> MAKDIEISASESKFILEALRQNYRLDGRSFDQFRDVEITFGKEFGDVSVKMGNTKVHCRISCQIAQPYEDRPFEGLFVISTEISPMAGSQFENGNITGEDEVLCSRIIEKSVRRSGALDVEGLCIVAGSKCWAVRADVHFLDCDGGFIDASCIAVMAGLMHFKKPDITVHGEQIIVHPVNEREPVPLGILHIPICVTFSFFNPQDTEENIKGETNSEISIIDATLKEELLRDGVLTVTLNKNREVVQVSKAGGLPMDALTLMKCCHEAYSIIEKITDQILQLLKEDSEKRNKYAAMLTSENAREI;> GHMSRLEIYSPEGLRLDGRRWNELRRFESSINTHPHAADGSSYMEQGNNKIITLVKGPKEPRLKSQMDTSKALLNVSVNITKFSKFERSKSSHKNERRVLEIQTSLVRMFEKNVMLNIYPRTVIDIEIHVLEQDGGIMGSLINGITLALIDAGISMFDYISGISVGLYDTTPLLDTNSLEENAMSTVTLGVVGKSEKLSLLLVEDKIPLDRLENVLAIGIAGAHRVRDLMDEELRKHAQKRVSNASAR;> MAESTTLETIEIHPITFPPEVLARISPELSLQRHLSLGIRPCLRKYEEFRDVAIENNTLSRYADAGNIDTKNNILGSNVLKSGKTIVITSITGGIIEETSASIKDLDDFGEEELFEVTKEEDIIANYASVYPVVEVERGRVGACTDEEMTISQKLHDSILHSRILPKKALKVKAGVRSANEDGTFSVLYPDELEDDTLNETNLKMKRKWSYVLYAKIVVLSRTGPVFDLCWNSLMYALQSVKLPRAFIDERASDLRMTIRTRGRSATIRETYEIICDQTKSVPLMINAKNIAFASNYGIVELDPECQLQNSDNSEEEEVDIDMDKLNTVLIADLDTEAEETSIHSTISILAAPSGNYKQLTLMGGGAKITPEMIKRSLLLSRVRADDLSTRFNI;> GHGNNKEPNTKNRLDSAEKKKKMSVQAEIGILDHVDGSSEFVSQDTKVICSVTGPIEPKARQELPTQLALEIIVRPAKGVATTREKVLEDKLRAVLTPLITRHCYPRQLCQITCQILESGEDEAEFSLRELSCCINAAFLALVDAGIALNSMCASIPIAIIKDTSDIIVDPTAEQLKISLSVHTLALEFVNGGKVVKNVLLLDSNGDFNEDQLFSLLELGEQKCQELVTNIRRIIQDNISPRLVV;> GHMSLSVAEKSYLYDSLASTPSIRPDGRLPHQFRPIEIFTDFLPSSNGSSRIIASDGSECIVSIKSKVVDHHVENELLQVDVDIAGQRDDALVVETITSLLNKVLKSGSGVDSSKLQLTKKYSFKIFVDVLVISSHSHPISLISFAIYSALNSTYLPKLISAFDDLEVEELPTFHDYDMVKLDINPPLVFILAVVGNNMLLDPAANESEVANNGLIISWSNGKITSPIRSVALNDSNVKSFKPHLLKQGLAMVEKYAPDVVRSLENL;> MNVQDRRRLLGPAAAKPMAFSNTTTHVPEKKSTDLTPKGNESEQELSLHTGFIENCNGSALVEARSLGHQTSLISAVYGPRSIRGSFTSQGTISIQLKNGLLEKYNTNELKEVSSFLMGIFNSVVNLSRYPKSGIDIFVYLTYDKDLTNNPQDDDSQSKMTSSQISSLIPHCITSITLALADAGIELVDMAGAGEANGTVVSFIKNGEEIVGFWKDDGDDEDLLECLDRCKEQYNRYRDLMISCLMNQET;> GPHMSTFIFPGDSFPVDPTTPVKLGPGIYCDPNTQEIRPVNTGVLHVSAKGKSGVQTAYIDYSSKRYIPSVNDFVIGVIIGTFSDSYKVSLQNFSSSVSLSYMAFPNASKKNRPTLQVGDLVYARVCTAEKELEAEIECFDSTTGRDAGFGILEDGMIIDVNLNFARQLLFNNDFPLLKVLAAHTKFEVAIGLNGKIWVKCEELSNTLACYRTIMECCQKNDTAAFKDIAKRQFKEILTVKEE;> RSMSEVITITKRNGAFQNSSNLSYNNTGISDDENDEEDIYMHDVNSASKSESDSQIVTPGELVTDDPIWMRGHGTYFLDNMTYSSVAGTVSRVNRLLSVIPLKGRYAPETGDHVVGRIAEVGNKRWKVDIGGKQHAVLMLGSVNLPGGILRRKSESDELQMRSFLKEGDLLNAEVQSLFQDGSASLHTRSLKYGKLRNGMFCQVPSSLIVRAKNHTHNLPGNITVVLGVNGYIWLRKTSQMDLARDTPSANNSSSIKSTGPTGAVSLNPSITRLEEESSWQIYSDENDPSISNNIRQAICRYANVIKALAFCEIGITQQRIVSAYEASMVYSNVGELIEKNVMESIGSDILTAEKMRGNGN;> GPHMACNFQFPEIAYPGKLICPQYGTENKDGEDIIFNYVPGPGTKLIQYEHNGRTLEAITATLVGTVRCEEEKKTDQEEEREGTDQSTEEEKSVDASPNDVTRRTVKNILVSVLPGTEKGRKTNKYANNDFANNLPKEGDIVLTRVTRLSLQRANVEILAVEDKPSPIDSGIGSNGSGIVAAGGGSGAATFSVSQASSDLGETFRGIIRSQDVRSTDRDRVKVIECFKPGDIVRAQVLSLGDGTNYYLTTARNDLGVVFARAANGAGGLMYATDWQMMTSPVTGATEKRKCAKPF;> GPAMSVPAIAPRRKRLADGLSVTQKVFVRSRNGGATKIVREHYLRSDIPCLSRSCTKCPQIVVPDAQNELPKFILSDSPLELSAPIGKHYVVLDTNVVLQAIDLLENPNCFFDVIVPQIVLDEVRNKSYPVYTRLRTLCRDSDDHKRFIVFHNEFSEHTFVERLPNETINDRNNRAIRKTCQWYSEHLKPYDINVVLVTNDRLNREAATKEVESNIITKSLVQYIELLPNADDIRDSIPQMDSFDKDLERDTFSDFTFPEYYSTARVMGGLKNGVLYQGNIQISEYNFLEGSVSLPRFSKPVLIVGQKNLNRAFNGDQVIVELLPQSEWKAPSSIVLDSEHFDVNDNPDIEAGDDDDNNESSSNTTVISDKQRRLLAKDAMIAQRSKKIQPTAKVVYIQRRSWRQYVGQLAPSSVD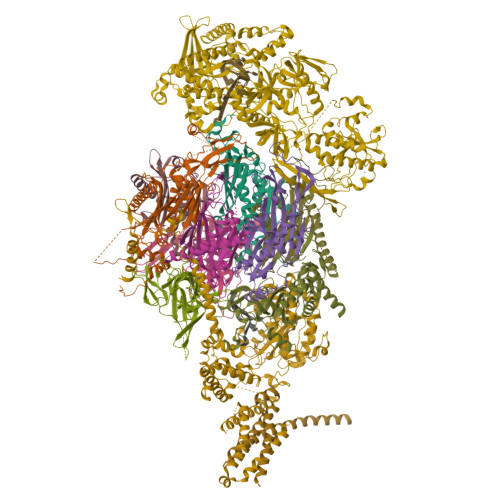PQSSSTQNVFVILMDKCLPKVRIRTRRAAELLDKRIVISIDSWPTTHKYPLGHFVRDLGTIESAQAETEALLLEHDVEYRPFSKKVLECLPAEGHDWKAPTKLDDPEAVSKDPLLTKRKDLRDKLICSIDPPGCVDINDALHAKKLPNGNWEVGVHIADVTHFVKPGTALDAEGAARGTSVYLVDKRIDMLPMLLGTDLCSLKPYVDRFAFSVIWELDDSANIVNVNFMKSVIRSREAFSYEQAQLRIDDKTQNDELTMGMRALLKLSVKLKQKRLEAGALNLASPEVKVHMDSETSDPNEVEIKKLLATNSLVEEFMLLANISVARKIYDAFPQTAMLRRHAAPPSTNFEILNEMLNTRKNMSISLESSKALADSLDRCVDPEDPYFNTLVRIMSTRCMMAAQYFYSGAYSYPDFRHYGLAVDIYTHFTSPIRRYCDVVAHRQLAGAIGYEPLSLTHRDKNKMDMICRNINRKHRNAQFAGRASIEYYVGQVMRNNESTETGYVIKVFNNGIVVLVPKFGVEGLIRLDNLTEDPNSAAFDEVEYKLTFVPTNSDKPRDVYVFDKVEVQVRSVMDPITSKRKAELLLK;> GAMASENPDVLLSRVINVVRAASSLASQDVDFYKNLDRGFSKDLKSKADKLADMANEIILSIDEHHESFELKEEDISDLWNNFGNIMDNLLEMSDHSLDKLNCAINSKSRGSDLQYLGEFSGKNFSPTKRVEKPQLKFKSPIDNSESHPFIPLLKEKPNALKPLSESLRLVDDDENNPSHYPHPYEYEIDHQEYSPEILQIREEIPSKSWDDSVPIWVDTSTELESMLEDLKNTKEIAVDLEHHDYRSYYGIVCLMQISTRERDYLVDTLKLRENLHILNEVFTNPSIVKVFHGAFMNIIWLQRDLGLYVVGLFDTYHASKAIGLPRHSLAYLLENFANFKTSKKYQLADWRIRPLSKPMTAYARADTHFLLNIYDQLRNKLIESNKLAGVLYESRNVAKRRFEYSKYRPLTPSSEVYSPIEKESPWKILMYQYNIPPEREVLVRELYQWRDLIARRDDESPRFVMPNQLLAALVAYTPTDVIGVVSLTNGVTEHVRQNAKLLANLIRDALRNIKNTNEEATPIPSSETKADGILLETISVPQIRDVMERFSVLCNSNISKSRAKPVTNSSILLGKILPREEHDIAYSKDGLPNKVKTEDIRIRAQNFKSALANLEDIIFEIEKPLVVPVKLEEIKTVDPASAPNHSPEIDNLDDLVVLKKKNIQKKQPAKEKGVTEKDAVDYSKIPNILSNKPG;> MEDIEKIKPYVRSFSKALDELKPEIEKLTSKSLDEQLLLLSDERAKLELINRYAYVLSSLMFANMKVLGVKDMSPILGELKRVKSYMDKAKQYDNRITKSNEKSQAEQEKAKNIISNVLDGNKNQFEPSISRSNFQGKHTKFENDELAESTTTKIIDSTDHIRKASSKKSKRLDKVGKKKGGKK> MLDAFSRAVVQADASTSVVGDVSALKQFIAQGNRRLDAVNAIASN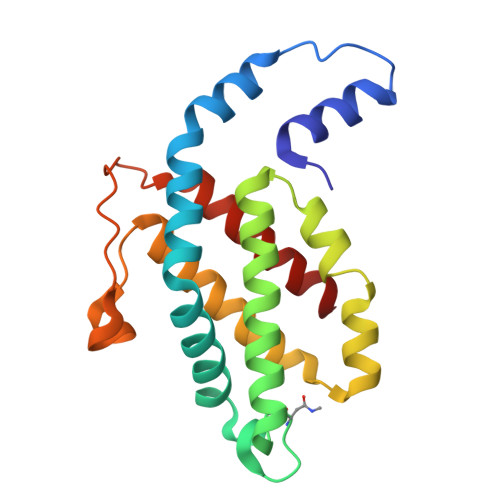ASCMVSDAIAGMICENQGLIQAGGNCYPNRRMAACLRDGEIILRYVTYALLAGDASVLDDRCLNGLKETYAALGVPTTSTVRAVQIMKAQAAAHIKDTPSEARAGAKLRKMGSPVVEDRCSSLVAEASSYFDRVIAALS> MTGHVSKTSHVPKGRPSSLAKKAAKRAMAKVNSNPKRASGHLERVVQSVNDATKRLSQPDSTVSVATKSSKRKSRDTVGPWKLGKTLGKGSSGRVRLAKNMETGQLAAIKIVPKKKAFVHCSNNGTVPNSYSSSMVTSNVSSPSIASREHSNHSQTNPYGIEREIVIMKLISHTNVMALFEVWENKSELYLVLEYVDGGELFDYLVSKGKLPEREAIHYFKQIVEGVSYCHSFNICHRDLKPENLLLDKKNRRIKIADFGMAALELPNKLLKTSCGSPHYASPEIVMGRPYHGGPSDVWSCGIVLFALLTGHLPFNDDNIKKLLLKVQSGKYQMPSNLSSEARDLISKILVIDPEKRITTQEILKHPLIKKYDDLPVNKVLRKMRKDNMARGKSNSDLHLLNNVSPSIVTLHSKGEIDESILRSLQILWHGVSRELITAKLLQKPMSEEKLFYSLLLQYKQRHSISLSSSSENKKSATESSVNEPRIEYASKTANNTGLRSENNDVKTLHSLEIHSEDTSTVNQNNAITGVNTEINAPVLAQKSQFSINTLSQPESDKAEAEAVTLPPAIPIFNASSSRIFRNSYTSISSRSRRSLRLSNSRLSLSASTSRETVHDNEMPLPQLPKSPSRYSLSRRAIHASPSTKSIHKSLSRKNIAATVAARRTLQNSASKRSLYSLQSISKRSLNLNDLLVFDDPLPSKKPASENVNKSEPHSLESDSDFEILCDQILFGNALDRILEEEEDNEKERDTQRQRQNDTKSSADTFTISGVSTNKENEGPEYPTKIEKNQFNMSYKPSENMSGLSSFPIFEKENTLSSSYLEEQKPKRAALSDITNSFNKMNKQEGMRIEKKIQREQLQKKNDRPSPLKPIQHQELRVNSLPNDQGKPSLSLDPRRNISQPVNSKVESLLQGLKFKKEPASHWTHERGSLFMSEHVEDEKPVKASDVSIESSYVPLTTVATSSRDPSVLAESSTIQKPMLSLPSSFLNTSMTFKNLSQILADDGDDKHLSVPQNQSRSVAMSHPLRKQSAKISLTPRSNLNANLSVKRNQGSPGSYLSNDLDGISDMTFAMEIPTNTFTAQAIQLMNNDTDNNKINTSPKASSFTKEKVIKSAAYISKEKEPDNSDTNYIPDYTIPNTYDEKAINIFEDAPSDEGSLNTSSSESDSRASVHRKAVSIDTMATTNVLTPATNVRVSLYWNNNSSGIPRETTEEILSKLRLSPENPSNTHMQKRFSSTRGSRDSNAL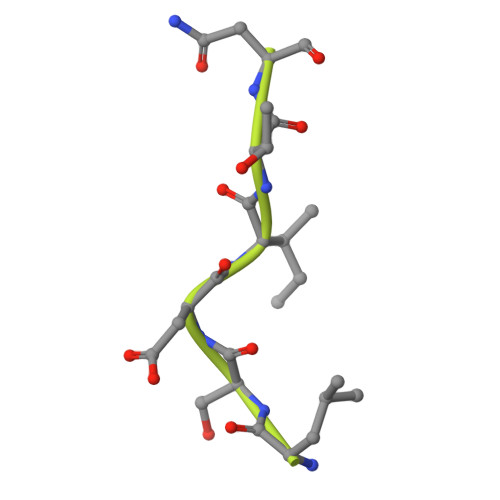GISQSLQSMFKDLEEDQDGHTSQADILESSMSYSKRRPSEESVNPKQRVTMLFDEEEEESKKVGGGKIKEEHTKLDNKISEESSQLVLPVVEKKENANNTENNYSKIPKPSTIKVTKDTAMESNTQTHTKKPILKSVQNVEVEEAPSSDKKNWFVKLFQNFSSHNNATKASKNHVTNISFDDAHMLTLNEFNKNSIDYQLKNLDHKFGRKVVEYDCKFVKGNFKFKIKITSTPNASTVITVKKRSKHSNTSSNKAFEKFNDDVERVIRNAGRS Here we elucidate the molecular basis of high-affinity phosphite and hypophosphite acquisition by determining the ligand-binding affinity and structure of the PBPs of phosphite and hypophosphite ABC transporters from environmental microorganisms. We over-produced and purified PBPs of three putative phosphite transporters; PtxB from the globally important marine diazotroph Trichodesmium erythraeum IMS101 (Te_PtxB), PhnD from the oceanic picocyanobacteria Prochlorococcus marinus MIT9301 (Pm_PhnD)35 and PtxB from the soil bacterium Pseudomonas stutzeri WM88 (Ps_PtxB), as well as a PBP from a putative hypophosphite transporter, HtxB, also from P. stutzeri WM88 (HtxB)18. The structures reveal that ligand specificity, measured here by thermophoresis, arises from a combination of steric considerations and the interaction between a ligand P-H hydrogen atom and an aromatic π system in the binding pocket. The structures of two distinct types of phosphite-binding protein and a hypophosphite-binding protein reveal that a P-H…π interaction ensures high-affinity binding of specific ligands, representing a universal mechanism in these PBPs for recognising ligands with a P-H bond.

Te_PtxB and Pm_PhnD have 2–4 orders of magnitude higher binding affinity for phosphite than phosphate and phosphonates, but whilst attempts to crystallise complexes of either protein with ethylphosphonate (EPn), 2AEPn or phosphate were unsuccessful, structures of both proteins in complex with methylphosphonate (MPn) were obtained. The overall fold of the Te_PtxB and Pm_PhnD complexes with MPn were very similar to the comparative complexes with phosphite (RMSD cα: ~0.3 Å) and since both MPn complexes were determined at high resolution (1.41–1.52 Å), the electron density for the ligand could be confidently interpreted within the binding pocket, with the MPn refining unequivocally in only one orientation. Given this similarity, it was unsurprising that the three oxygen atoms and the phosphorus atom of the MPn bind in the same position as those of the phosphite, with the methyl group of the MPn pointing in the same direction as the R1 hydrogen of the phosphite, towards the capping tyrosine residue (Y208/Y206). To accommodate the methyl group of the MPn the tyrosine moves in both structures by ~0.5 Å, compared to the complexes with phosphite, resulting in an ~16% expansion in the volume of the binding pocket. Despite this movement, the methyl-carbon atom of the MPn lies ~3.0 Å from the plane of the tyrosine ring in both structures. This might suggest that a C-H…π interaction is present, however the relative geometry of the two partners is sub-optimal for this type of interaction. Thermal ellipsoids were calculated from the anisotropic B-factors for the three structures that were better than 1.5 Å resolution (Te_PtxB and Pm_PhnD with MPn and Pm_PhnD with phosphite).

>[2x]MNIQKSENKANPQKLVVALLPDESAATVIQNNKGLEMYLENKLNKDIELFVSTDYSSMIEVASKGRLDLAYFGPLSYVLAKTKSNIEPFAALEKDGKNTYQALVIGNAEAGINSYEKIEGKIMAYGDQASTSSHLIPKSMLKQKQLKAGENYEEVFVGAHDAVAIAVANGKAQAGGLSKPIFTALIERGTIDKNKVIIIAESKPFPQYPWTMRSDLDSELKTQIQQAFLELEDKAILKPFKADAFTLVTDQDYDVVRNLGEVLELNFEQLNKLEHHHHHH> AVSLDRTRAVFDGSEKSMTLDISNDNKQLPYLAQAWIENENQEKIITGPVIATPPVQRLEPGAKSMVRLSTTPDISKLPQDRESLFYFNLREIPPRSEKANVLQIALQTKIKLFYRPAAIKTRPNEVWQDQLILNKVSGGYRIENPTPYY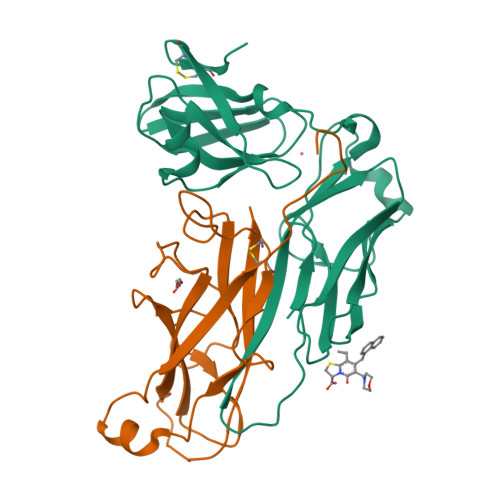VTVIGLGGSEKQAEEGEFETVMLSPRSEQTVKSANYNTPYLSYINDYGGRPVLSFICNGSRCSVKKEK;> GPFPPPGMSLPEYWGEEHVWWDGRAAFHGEVVRPACTLAMEDAWQIIDMGETPVRDLQNGFSGPERKFSLRLRNCEFNSQGGNLFSDSRIRVTFDGVRGETPDKFNLSGQAKGINLQIADVRGNIARAGKVMPAIPLTGNEEALDYTLRIVRNGKKLEAGNYFAVLGFRVDYE beta-L-arabinopyranose | C5 H10 O5 | 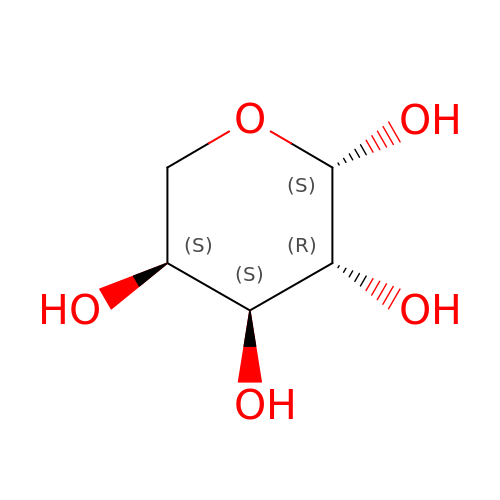SRBFZHDQGSBBOR-KLVWXMOXSA-N> EARLEEAVNRWVLKFYFHEALRAFRGSRYGDFRQIRDIMQALLVRPLGKEHTVSRLLRVMQCLSRIEEGENLDCSFDMEAELTPLESAINVLEMIKTEFTLTEAVVESSRKLVKEAAVIICIKNKEFEKASKILKKHMSKDPTTQKLRNDLLNIIREKNLAHPVIQNFSYETFQQKMLRFL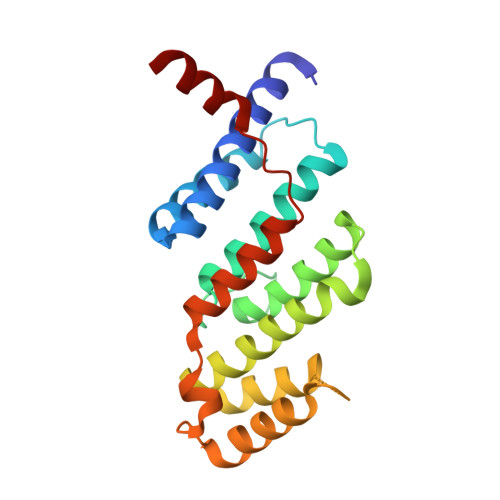ESHLDDAEPYLLTMAKKAL>MRSMSELIVSRQQRVLLLTLNRPAARNALNNALLMQLVNELEAAATDTSISVCVITGNARFFAAGADLNEMAEKDLAATLNDTRPQLWARLQAFNKPLIAAVNGYALGAGCELALLCDVVVAGENARFGLPEITLGIMPGAGGTQRLIRSVGKSLASKMVLSGESITAQQAQQAGLVSDVFPSDLTLEYALQLASKMARHSPLALQAAKQALRQSQEVALQAGLAQERQLFTLLAATEDRHEGISAFLQKRTPDFKGR[2x];>MGSSHHHHHHGSMMEFILSHVEKGVMTLTLNRPERLNSFNDEMHAQLAECLKQVERDDTIRCLLLTGAGRGFCAGQDLNDRN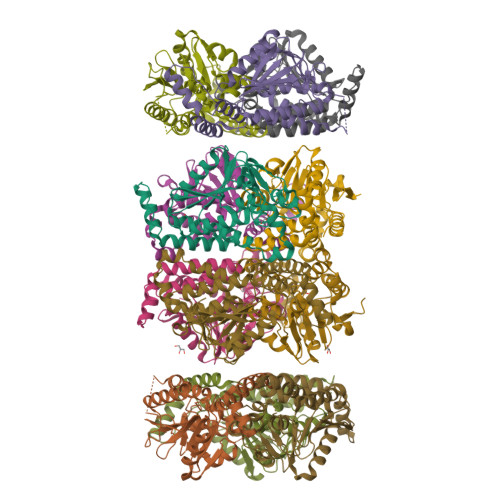VDPTGPAPDLGMSVERFYNPLVRRLAKLPKPVICAVNGVAAGAGATLALGGDIVIAARSAKFVMAFSKLGLIPDCGGTWLLPRVAGRARAMGLALLGNQLSAEQAHEWGMIWQVVDDETLADTAQQLARHLATQPTFGLGLIKQAINSAETNTLDTQLDLERDYQRLAGRSADYREGVSAFLAKRSPQFTGK[2x]> ADQKLSDFHAESGGCESCHKDGTPSADGAFEFAQCQSCHGKLSEMDAVHKPHDGNLVCADCHAVHDMNVGQKPTCESCHDDGRT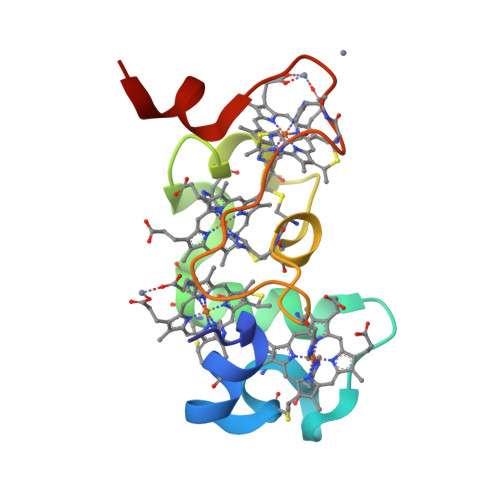SASVLKK>[2x]MAHHHHHHMEHNYFYKNSATLKNKHGIKNPRKLYERCAHETA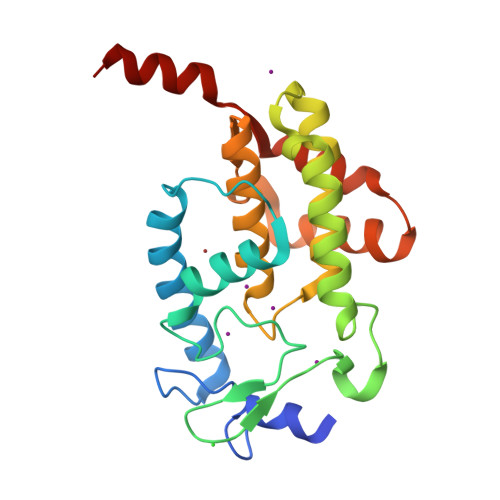REAVNFRLEPPPGKFDAAYLRTIHWCLFHNTFEWAGVTRDQPFTFEDGSTACMPAMRPKGYKVPFAVGSQIQRELKKLEQRLTAKNNLQGLSRQEFAANAAEVFTALDHAHPFRKGNGRTQRMFMEKLGQAAGYKIDFSLITKERMTYASIEAMQHNNPEPMKDLFEDITHPQKSLLLKEFISQM DSR2, a Sir2 domain-containing protein, protects bacteria from phage infection by hydrolyzing NAD+. The enzymatic activity of DSR2 is triggered by the SPR phage tail tube protein (TTP), while suppressed by the SPbeta phage-encoded DSAD1 protein, enabling phages to evade the host defense. The protomer structure of DSR2 revealed an architecture that consists of an N-terminal Sir2 domain (residues 1–298) and a long C-terminal helical region (residues 299–1005). The Sir2 domains of two side-by-side DSR2 dimers contact each other to assemble into a head-to-head rod-shaped homo-tetramer of DSR2.

The gel filtration profile shows that the DSR2 tends to form large oligomers. To further investigate the mechanism of DSR2 oligomerization and NAD+ binding, we collected the cryo-EM dataset of DSR2 H171A catalytically inactive mutant, and determined the cryo-EM structure of DSR2 (H171A) to overall 3.18 Å resolution. The resolution of central part of DSR2 structure is better than 3 Å, and that of the very C-terminal region is relatively poor due to the dynamic property which was indicated by the local resolution maps and 3D variability analysis. The overall structure, especially the two ends, undergoes continuous motion. Local refinement focused on the C-terminus of DSR2 improved the resolution, which allowed us to construct the atomic model and precisely assign the sidechain orientations, assisted by AlphaFold2 predicted model. Interestingly, the two side-by-side DSR2 molecules form an asymmetric dimer, with the one cavity at DSR2 C-terminus closed while the other partially opened. Comparing these two cavities, we observed the structures of the C-terminal domains of two DSR2 protomers are distinct. The C-terminal domain with opened cavity rotates upward and thus moves away from the cavity center compared to the closed one. Additionally, a long helix in R1 of the HEAT repeat domain of one DSR2 protomer with a partially opened cavity directly contacts the C-terminal domain from the other protomer, which facilitates the closure of its C-terminal cavity. The interface 1 consists of the contacts between the last two α-helices from the C-terminal domains of two adjacent DSR2 molecules. This interface is primarily maintained through hydrophobic interactions, wherein the hydrophobic side chains of I981, V988, L997, L1000, M1001, and L1005 from two DSR2 protomers form extensive hydrophobic interactions with one another.

>[2x]MVKVDLESKRYGEKLKEVFLMLDNNVVECIKEITESSRNGKLVFFVGAGVSTLSDYPQWWRLVDKYHEELYGSPKKGNYSSDEYLRIPQIFYNVKGEMAFDGILKDFFQVDKPTNPIHDKILAMNPAHVITTNYDNLIDTACWKRGKYFSVISAEEDVANATSSRYLLKVAGDFRKGFKGENVVLKEDDYLNYDQNYPLISNLMKTIIATHTIVFIGYGLGDYNINMLLNWVRKLQKDSFHKPFFIRTDPSPIENETLIYYENKGLRIIDAASLIDSNEYDYLERYSAVMDLLIESQENKFITKDDEVIDYIYGKISPLFALQYIRKIDLKHVFEYDYHFEVNGTVVRHKNKGFGYMERFFELKESCDERSKLSKKQYERFNALFNFFEKNGVICMAKDAGTLNTSIEINSLAYHGKYDVMKKFIEEQSVSIEDDYKKAFFLACLGRWEESYDLYSNIILNSIDESNGCVYYLSQINRYRIYQSITQAVTQFNGLGLLTFGRHYKPFTDEFLARIEREMTNFNIDDLFNGMPFEFQKKYKILEFLSDNQFLYDDTVKLFELTNKVRSEMSEGSYSFGMSSDIVVLLRLYDNLRFLYENCLWSVSFHEFHQYIRNSMSLLIEKAEYERTRDIDELGFSFFGKKSGFFMEYYDFVNISRHFKIDDIKNLERSCSIDKIRFGEQEKIEEYLVGIAEEITKQFSANGMNVVFYTQFISEAKAALYFAKYVKLSEEGLGKIVKALLFYFPERDLDIGKRYVWLERLTKCNELPKSIISIIDDFLVLQAEKHIDQNYSEVSSNGLYSRDYGALIKHFEKNFISKRLSEITLCLTQDKQKQIDFLFKLLPLLSTNAKSHLLSFKSVENINDLMNGIRIGLIDEFTPEHEELIIEYLETRKVNYIVEKEKGIQTFSSNDYMSTFGIWYFLEEINNSKMEEFIGMDDQYDFFVDPENFDYKKFIPSWLKNYNDKLLGKIAGNKHMKHHVIEVLKERVKNSNDKRYLEILMNYFI> SSLDDKPQFPGASAEFIDKLEFIQPNVISGIPIYRVMDRQGQIINPSEDPHLPKEKVLKLYKSMTLLNTMDRILYESQRQGRISFYMTNYGEEGTHVGSAAALDNTDLVFGQYREAGVLMYRDYPLELFMAQCYGNISDLGKGRQMPVHYGCKERHFVTISSPLATQIPQAVGAAYAAKRANANRVVICYFGEGAASEGDAHAGFNFAATLECPIIFFCRNNGYAISTPTSEQYRGDGIAARGPGYGIMSIRVDGNDVFAVYNATKEARRRAVAENQPFLIEAMTYAIGHASTSDDSSAYRSVDEVNYWDKQDHPISRLRHYLLSQGWWDEEQEKAWRKQSRRKVMEAFEQAERKPKPNPNLLFSDVYQEMPAQLRKQQESLARHLQTYGEHYPLDHF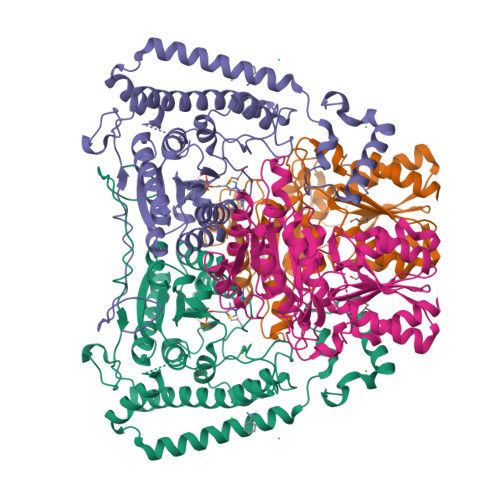DK;> VAHFTFQPDPEPREYGQTQKMNLFQSVTSALDNSLAKDPTAVIFGEDVAFGGVFRCTVGLRDKYGKDRVFNTPLCEQGIVGFGIGIAVTGATAIAEIQFADYIFPAFDQIVNEAAKYRYRSGDLFNCGSLTIRSPWGCVGHGALYHSQSPEAFFAHCPGIKVVIPRSPFQAKGLLLSCIEDKNPCIFFEPKILYRAAAEEVPIEPYNIPLSQAEVIQEGSDVTLVAWGTQVHVIREVASMAKEKLGVSCEVIDLRTIIPWDVDTICKSVIKTGRLLISHEAPLTGGFASEISSTVQEECFLNLEAPISRVCGYDTPFPHIFEPFYIPDKWKCYDALRKMINY> MYVYKRDGRKEPVQFDKITARISRLCYGLDPKHIDAVKVTQRIISGVYEGVTTIELDNLAAETCAYMTTVHPDYATLAARIAISNLHKQTTKQFSKVVEDLYRYVNAATGKPAPMISDDVYNIVMENKDKLNSAIVYDRDFQYSYFGFKTLERSYLLRINGQVAERPQHLIMRVALGIHGRDIEAALETYNLMSLKYFTHASPTLFNAGTPKPQMSSCFLVAMKEDSIEGIYDTLKECALISKTAGGIGLHIHNIRSTGSYIAGTNGTSNGLIPMIRVFNNTARYVDQGGNKRPGAFALYLEPWHADIFDFIDIRKNHGKEEIRARDLFPALWIPDLFMKRVEENGTWTLFSPTSAPGLSDCYGDEFEALYTRYEKEGRGKTIKAQKLWYSILEAQTETGTPFVVYKDACNRKSNQKNLGVIKSSNLCCEIVEYSAPDETAVCNLASVALPAFIETSEDGKTSTYNFKKLHEIAKVVTRNLNRVIDRNYYPVEEARKSNMRHRPIALGVQGLADTFMLLRLPFDSEEARLLNIQIFETIYHASMEASCELAQKDGPYETFQGSPASQGILQFDMWDQKPYGMWDWDTLRKDIMKHGVRNSLTMAPMPTASTSQILGYNECFEPVTSNMYSRRVLSGEFQVVNPYLLRDLVDLGIWDEGMKQYLITQNGSIQGLPNVPQELKDLYKTVWEISQKTIINMAADRSVYIDQSHSLNLFLRAPTMGKLTSMHFYGWKKGLKTGMYYLRTQAASAA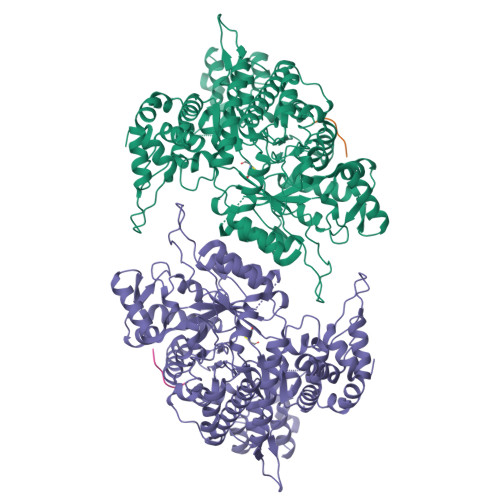IQFTIDQKIADQATENVADISNLKRPSYMPSSASYAASDFVPAAVTANATIPSLDSSSEASREASPAPTGSHSLTKGMAELNVQESKVEVPEVPAPTKNEEKAAPIVDDEETEFDIYNSKVIACAIDNPEACEMCSG;> KEINFDDDF>[3x]HHHHHHSSGMASINLPFSLSGSKRIPTSEELADGYQCGPLDVELDNWLMWWLTGQVDGVIEGAGLTTDDTDLARLYKAIQSMTSGNLRTVVLTAASGNLPIPSDVSVLNWVRAVGGGGAGGNSNTGNSKASGGGGGAGFDRFNVAVTPGSNVPYTVGAAGAVNGLGAGYNGGAGGSTAILGTTAGGGAGGLGVNNNATAVQVNGGTTSGTTPEISYPGGLGTEGIVGTGGGSVLSQPTQRAFTNAGNNNPANSWGGGGPGGSDFGGAWQPGGVGKQGIIIVQYFSRFAP;>MTDKHYARVVDGLVVETKTLPADFNLDDLFGPDHGWVEAPLEVEQGWRKVGAKFAPAPPPERDPASILAGLKAEASRHIFATISATAQSNLLLAVGLASAKAPSARTPEERDLLNVADEGRAWIDAVRARVHALAEHDGVTPKGEDRWPAPSEAVLEMAAKF[3x]

Pam3 has a minimal baseplate of only six protein components, and it possesses a much simpler tail fiber composed of only one protein gp24, providing an ideal model for synthetic engineering and biotechnological applications. Here, using a minimal myocyanophage, termed Pam3, isolated from Lake Chaohu, we demonstrate that the chaperone gp25 forms a stable complex with the tail fiber gp24 at a stoichiometry of 3:3. Each gp24 subunit consists of three domains: the N-terminal α-helical domain required for docking to the baseplate, the tumor necrosis factor (TNF)-like and glycine-rich domains responsible for recognizing the host receptor. Each gp25 subunit consists of two domains: a non-conserved N-terminal β-sandwich domain that binds to the TNF-like and glycine-rich domains of the fiber, and a C-terminal α-helical domain that mediates trimerization/assembly of the fiber.

To gain structural insights into gp25-assisted assembly of gp24 trimer, we determined the cryo-EM structure of the gp24-gp25 complex at 3.1 Å resolution. The residues from Leu31 to Pro280 of gp24 were modeled to the final structure. By contrast, the structure of the full-length gp25 (residues Met1~Phe162) was solved. In the gp24-gp25 complex, the gp24 trimer adopts an extended structure, whereas three separated β-sandwich domains of gp25 trimer embrace the distal moieties of gp24 trimer at the center, forming an elongated complex structure of ~140 Å in length. Seeing along the three-fold axis, the gp25 trimer covers the distal loops of gp24, making these loops inaccessible to the solvent. These loops located at the distal of tail fiber were proposed to recognize the host; thus, the chaperone gp25 should be released prior to the maturation of viral particles. Compared to the loose contact within the pairwise TNF-like domain and glycine-rich domain, extensive hydrophobic interactions in the N-terminal α-helical bundle contribute the majority to the trimerization of gp24. Each loop has two glycine-rich motifs (GRMs) that adopt an elongated conformation. These loops run parallel to the fiber axis and stack together into a four-layer lattice at an interval distance of ~5 Å (calculated from Cα atoms) between adjacent GRMs. By contrast, the three β-sandwich domains are separated from each other, which individually protrude outwards like three “tentacles” to stick onto the junction between C-terminal TNF-like and glycine-rich domains of gp24 trimer. The β-sandwich domain of one gp25 subunit interacts with the surface-exposed regions at the lateral of the TNF-like and glycine-rich domains of one gp24 subunit, forming an interface area of ~550 Å2.> MAKVRIYQLAKELGMETQELLELLDQMGVAYKSHASTLEEKDAEAVRELVKEQRGLQEKLAEEERRKSLPRRPPVVVIMGHVDHGKT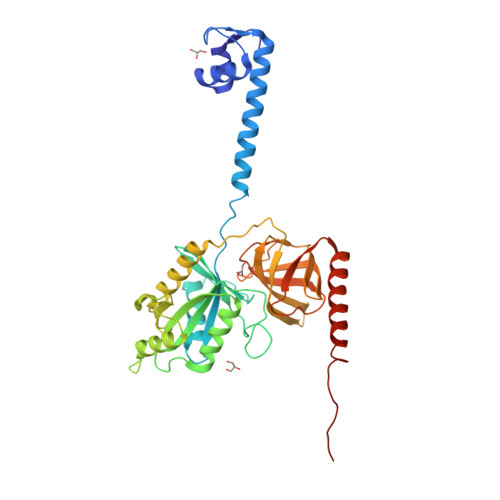TLLDYLRKSRIAEKEGGGITQHVGAFEVKTPQGTVVFIDTPGHEAFTTIRQRGAKVADIAVIVIAADDGIMPQTEEAIAHAKAAGAKLIFAINKIDLPQADPEKVKRQLMERGFVPEEYGGDAIVIPISAKTGQGVQDLLEMILLLAELEDYRADPNAEPRGVILESKLDKQAGIIANMLVQEGTFRVGDYVVAGEAYGRIRAMMDADGNQRKEAGPGSAVQVLGFQELPHAGDVVEWVPDLEAAKEIAEERKEERKAREEEEKARRPRTMAELLR>GTGDGSMSTPAPAFDRDQILLHLSLLRKDIATTRYRAIWPRREDKVKAWTTPLTGATVQDAVTQGFNSYIVVGDGGDSDAEITSVNAIFGEWDDGDLAWQVGAWEACGLPRPSFQLRTGGKSIHHYWVFHSPVDVPAWTELQARLIALAGFDTTNRNPSRVMRLAGCPHQRTGEVAQIFNATGELYDPGQMLQVLP[2x]

Among them, cyanophage S-2L is unique because its genome has all its adenines (A) systematically replaced by 2-aminoadenines (Z). Here, we identify the enzyme that is responsible for genome duplication of the phage S-2L, a member of the PrimPol family, and we present its crystal structure. We confirm its polymerase activity but find that the enzyme is not specific to A or Z. Instead, we propose that the absence of A in S-2L genome is explained by a separate enzyme, an HD phosphohydrolase that specifically dephosphorylates dATP and that we name DatZ. We give a structural explanation for both the specificity and the reaction mechanism of DatZ, based on three crystallographic structures, including one determined at sub-angstrom resolution.

The first region (1–190) corresponds to the AEP domain itself, with all crucial motifs conserved. Ca2+ ions were mandatory in the mother liquor to obtain crystals. As expected, the protein has a classical AEP fold. All crucial residues cluster together in the catalytic site of the domain. Y63, E85, D87, T112, K115, H118, D146, R157 are conserved across all AEPs (or have biochemically similar counterparts), and their function is well established in the superfamily. Residues E85, D87 (that can vary to Asp and Glu, respectively) coordinate a divalent metal ion (M2+) in the B site, that positions the triphosphate of the incoming nucleotide (dNTP) during polymerisation; this triphosphate is further stabilised by interactions with T112, K115, H118 and R157 (possibly varying respectively to Ser, Arg, Asn and Lys). Residue D146 along with residues E85, D87 and the dNTP’s α-phosphate coordinate another M2+ ion in the A site, making it possible to add the incoming dNTP to the primer strand of the nascent nucleic acid through the two-metal-ion mechanism. Importantly, in S-2L PP-N190 we noticed a significant positional shift of residue D87 compared to other AEP structures, along with the conservation among the close relatives of the neighbouring residue D88, which is exposed to the solvent. In all cases, the catalytic site is open to the solvent and there is no selection on the incoming nucleotides; after superposition with these structures, PP-N190 presents no structural feature that could lead to a Z vs A specificity during the polymerase reaction. Due to the presence of divalent calcium ions in all crystallisation conditions, we could not soak the crystals with nucleotides which immediately precipitate; transferring crystals to a solution devoid of Ca2+ dissolved them in a matter of seconds.> ASWIKEGELSLWERFCANIIKAGPMPKHIAFIMDGNRRYAKKCQVERQEGHSQGFNKLAETLRWCLNLGILEVTVYAFSIENFKRSKSEVDGLMDLARQKFSRLMEEKEKLQKHGVCIRVLGDLHLLPLDLQELIAQAVQATKNYNKCFLNVCFAYTSRHEISNAVREMAWGVEQGLLDPSDISESLLDKCLYTNRSPHPDILIRTSGEVRLSDFLLWQTSHSCLVF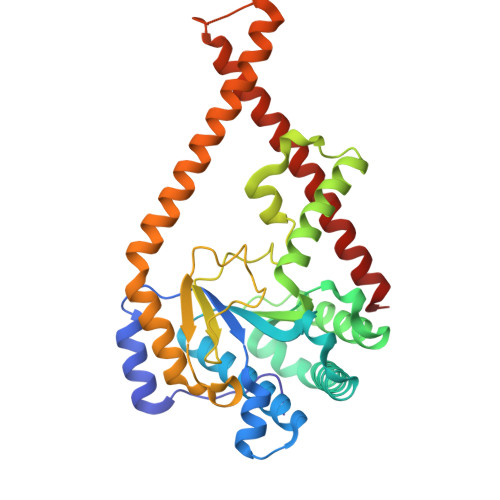QPVLWPEYTFWNLFEAILQFQMNHSMLQKARDMYAEERKRQQLERDQATVTEQLLREGLQASGDAQLRRTRLHKLSARREERVQGFLQALELKRADWLARLGT(3R,4S)-1-(3,4-DIMETHOXYPHENYL)-3-(3-METHYLPHENYL)PIPERIDIN-4-AMINE | 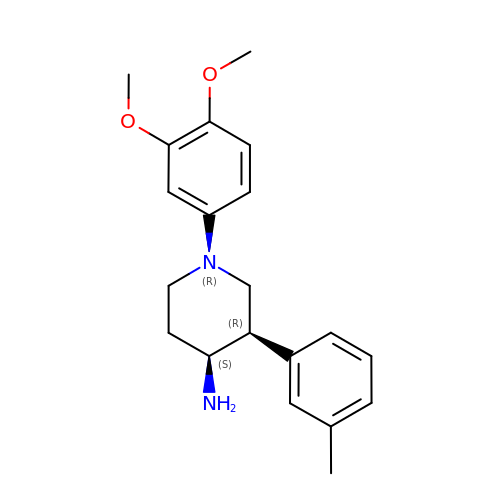C20 H26 N2 O2 | DQJXBZGPJVSWFI-ROUUACIJSA-N>[2x]MHHHHHHVNSLEMLTAIDYLTKKGWKISSDPRTYDGYPKNYGYRNYHENGINYDEFCGGYHRAFDVYSNET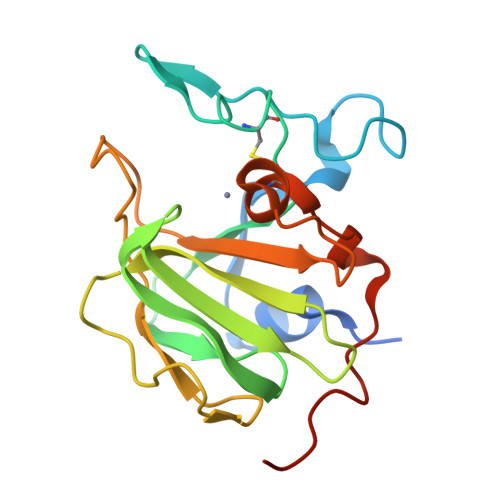NDVPAVTSGTVIEANDYGNFGGTFVIRDANDNDWIYGHLQRGSMRFVVGDKVNQGDIIGLQGNSNYYDNPMSVHLHLQLRPKDAKKDEKSQVCSGLAMEKYDITNLNAKQDKSKN>MMVLRMKVEWYLDFVDLNYEPGRDELIVEYYFEPNGVSPEEAAGRIASESSIGTWTTLWKLPEMAKRSMAKVFYLEKHGEGYIAKIAYPLTLFEEGSLVQLFSAVAGNVFGMKALKNLRLLDFHPPYEYLRHFKGPQFGVQGIREFMGVKDRPLTATVPKPKMGWSVEEYAEIAYELWSGGIDLLKDDENFTSFPFNRFEERVRKLYRVRDRVEAETGETKEYLINITGPVNIMEKRAEMVANEGGQYVMIDIVVAGWSALQYMREVTEDLGLAIHAHRAMHAAFTRNPRHGITMLALAKAARMIGVDQIHTGTAVGKMAGNYEEIKRINDFLLSKWEHIRPVFPVASGGLHPGLMPELIRLFGKDLVIQAGGGVMGHPDGPRAGAKALRDAIDAAIEGVDLDEKAKS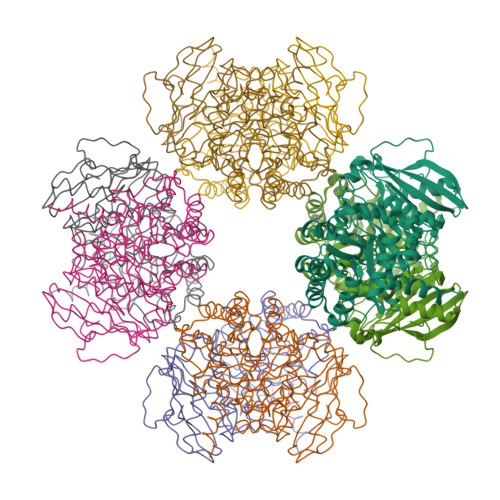SPELKKSLREVGLSKAKVGVQH[4x]>MKLSARNQLAGKVVSIKEGAVNGIVVLDIGGGNQISSTISMDSIRELGLQVGSDAYAVIKATSVMIGIDDWSHPQFEK[12x]

Here, we characterized E. limosum Tub, a tungsten storage protein. Tub has a sub-nanomolar affinity for tungstate and contains a single TOBE domain first characterized in a molybdate storage protein. Crystal structures revealed Tub assembles as a hexamer composed of a trimer of dimers, capable of binding eight tungstate oxyanions at two distinct binding sites located at inter-subunit interfaces. Tub enables E. limosum to accumulate W and then supplies W for two tungstoenzymes needed for conversion of lactate to SCFAs.

Isothermal titration calorimetry (ITC) analysis revealed that Tub contains two different binding sites for tungstate. Their individual binding properties could not be determined and the estimated Ka value was 1.00 pM with a saturating molar ratio of W to Tub of 1.44 ± 0.04:1. rTub was resistant to trypsin digestion both with and without added tungstate but was converted to the trypsin-sensitive monomeric form by TCA treatment. Similarly, Mo-loaded Tub exhibited the same thermal stability as the W-loaded form and was also resistant to trypsin digestion. In all crystal structures, three copies of the Tub dimer are arranged around a non-crystallographic threefold axis to form a spherical hexamer of 32 symmetry of 45 Å in diameter.> GTTAKQAEAVEDSDINPWTGQRHSERYFKILKARRKLPVNKQRQEFLDLYHNNQILVFVGETGSGKTTQIPQYVLYDELPHQTGKLIACTQPRRVAAMSVAQRVADELDVKLGEEVGYSIRFENKTSSKTLLKYMTDGQLLREAMHDRDMSRYSCIILDEAHERTLATDILMALLKQLSERRKDLKIIVMSATLDAQKFQSYFFNAPLLAVPGRTHPVEIFYTPEAERDYVEAAIRTVLQIHACEPEGDILLFLTGEEEIEDACRRISLEVDEMIRESDAGPMSVYPLYGTLPPHQQQRIFEKAPQPFRPGGRPGRKCIVATNIAETALTIDGIVYVVDPGFSKQKIYNPRTRVESLLVSPISKASAQQRAGRAGRTRPGKCFRLYTEEAFKKELIEQTYPEILRSNLSNTVLELKKLGVEDLVHFDLMDPPAPETMMRALEELNYLACLDDDGELTPLGNLASEFPLDPALAVMLISSPEFYCSNEILSITSLLSVPQIWVRPANARKRADEMKAQFAHPDGDHLTLLNAYHAYKGAEARGEDMKKWCHEHFLSYRHLSSADNVRAQLKKIMETHGIELVSTPFHDKNYYTNIRRALLAGFFMQVAMRESSNSKVYKTVKDEQLVLIHPSTTVTTPYEWVVYNEFVLTTKQYVRTVTNIRPEWLLEIAPVYYDLSTFQKGEIKNALTRVAEKIRRQQAMKASKA

DEAH-box adenosine triphosphatases (ATPases) play a crucial role in the spliceosome-mediated excision of pre-mRNA introns. The catalytic activation, the catalysis itself as well as the final disassembly steps are driven by so-called DEAH-box helicases. They all belong to the helicase superfamily 2 (SF2) and share at least eight conserved sequence motifs (motifs I, Ia, Ib, II, III, IV, V and VI) spread over two RecA-like domains that together form the helicase core. Two RecA-like domains, referred to as RecA1 and RecA2, build up the helicase core. The RecA2 domain contains an anti-parallel β-hairpin present in all DExH-box helicases, which protrudes out of the RecA2 domain thereby contacting the C-terminal domains. These domains are divided in three distinct domains, namely the winged-helix (WH), the helix-bundle (HB) and the oligonucleotide-binding (OB) domain.

A structural analysis revealed that a serine in motif V is involved in polar interactions with one of the ligands in all structurally characterized catalytic states. We could furthermore structurally characterize Prp22-S837A in the adenosine nucleotide-free but RNA-bound state, as well as Prp43-S387A and Prp43-S387G in the ATP-bound state. Since Prp22 could not be crystallized in the presence of an ATP-analog, an existing crystallization condition for ADP-BeF3−-bound Prp43 was used to structurally characterize motif V serine mutants of a DEAH-box ATPase in this state. The structures of these three mutants show that motif V is able to adopt the same nucleotide-specific conformations regardless of the side chain property. In the ADP/ATP-bound structures, the mainchain of this residue interacts via hydrogen-bonds with conserved water molecules constituting the active site. The side chain of the serine additionally interacts with another water molecule and two active site residues when ATP is present. The interactions in the ATP-bound state force the serine mainchain to adopt an unfavored conformation, enabling the mainchain nitrogen to hydrogen bond with the catalytic water. As a consequence, the C-terminus of the motif V helix is disrupted. Summarizing our data show that the serine side chain is dispensable for the function of motif V and instead has a regulatory role. Instead, the mainchain is sufficient for sensing the adenosine nucleotide state at the active site and this sensing function is sensitive to the flexibility of the mainchain.> MTEYIQDAIPAKLAIAIANPIFPQLDSQLRAGRHISIEMLDEHAFLMDFQTELESFYRRYHVDL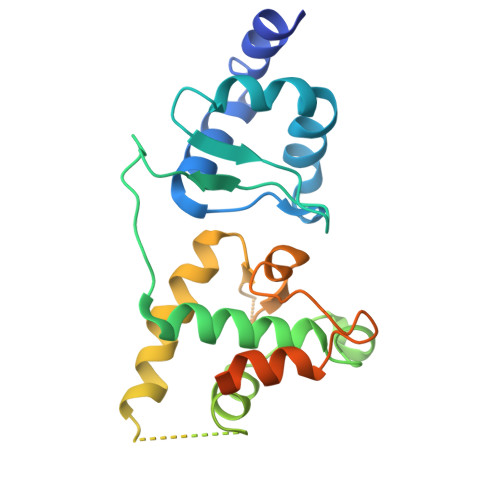IRAPEGFFYLRPKASTLIARSAMSEMEMLVGKVLCYLYLSPERLAQQGIFSQDDVYEELLNLADENKLLKAVNPRSTGSDLDRAKLAEKVGGALRRLARIGIITRVGEQNSKKFIISEAVFRFGADVRAGDDPREVQLRLIRDGEATTPTLLTTAAIEFAEDGARDELEESEAE> QYAPQTQSGRTSIVHLFEWRWVDIALECERYLGP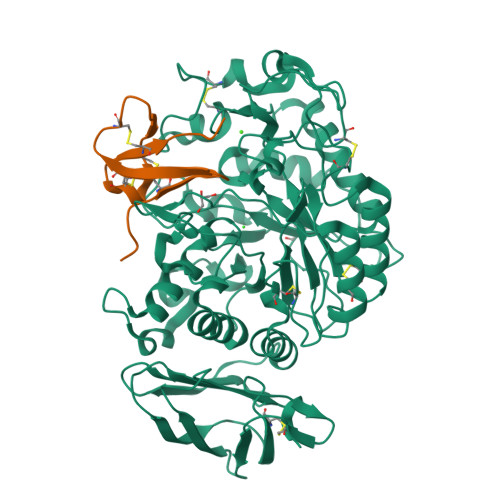KGFGGVQVSPPNENVVVTNPSRPWWERYQPVSYKLCTRSGNENEFRDMVTRCNNVGVRIYVDAVINHMCGSGAAAGTGTTCGSYCNPGSREFPAVPYSAWDFNDGKCKTASGGIESYNDPYQVRDCQLVGLLDLALEKDYVRSMIADYLNKLIDIGVAGFRIDASKHMWPGDIKAVLDKLHNLNTNWFPAGSRPFIFQEVIDLGGEAISSSEYFGNGRVTEFKYGAKLGTVVRKWSGEKMSYLKNWGEGWGFMPSDRALVFVDNHDNQRGHGAGGSSILTFWDARLYKVAVGFMLAHPYGFTRVMSSYRWARNFVNGEDVNDWIGPPNNNGVIKEVTINADTTCGNDWVCEHRWREIRNMVWFRNVVDGQPFANWWDNGSNQVAFGRGNRGFIVFNNDDWQLSSTLQTGLPGGTYCNVISGDKVGNSCTGIKVYVSSDGTAQFSISNSAQDPFIAIHAESKL;> ESGNSCYIYHGVSGICKASCAEDEKAMAGMGVCEGHLCCYKTPW>XEVYKLDANVKRLEKEV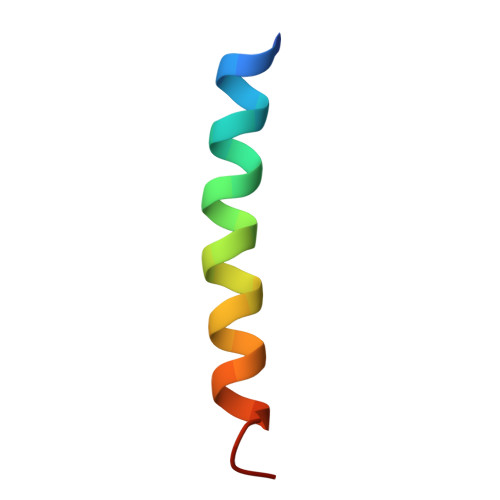GKLEGEVARLX[4x]> MNTLKSLRTTFLEELKSKVTATEPAGLYDPVHYILDLGGKRLR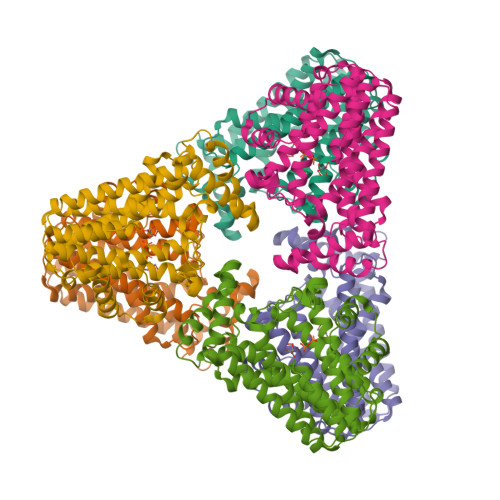PLLTLMSAEMYGATAKDAMNAAIAVEVFHNFTLLHDDIMDAADLRRGKETVHKKWDVNTGILTGDAMLIMAYRLFEDYDKDKFYQLNKVFSRTALEVCEGQQHDVDFETRDDVSVPEYLNMIKLKTSVLVGCALQMGAIIAGVDEKEQELIYDYGINLGLAFQLMDDYLDAFGDPETFGKEVGGDIRENKKTYLYLKSIENNDCATELKEWFALHFENMTEEQIDEKKETVKVFFEQSGGAKATLDAIESYTQKALKNIEELSIAPESKKQLTDFSLQLMGRKSLEHHHHHH>MATTVQLSDQSLRQLETLAIHTAHLIQPHGLVVVLQEPDLTISQISANCTGILGRSPEDLLGRTLGEVFDSFQIDPIQSRLTAGQISSLNPSKLWARVMGDDFVIFDGVFHRNSDGLLVCELEPAYTSDNLPFLGFYHMARAALNRLRQQANLRDFYDVIVEEVRRMTGFDRVMLHRFDENNHGDVIAEDKRDDMEPYLGLHYPESDIPQPARRLFIHNPIRVIPDVYGVAVPLTPAVNPSTNRAVDLTESILRSAYHCHLTYLKNMGVGASLTISLIKDGHLWGLIACHHQTPKVIPFELRKACEFFGRVVFSNISAQEDTETFDYRVQLAEHEAVLLDKMTTAADFVEGLTNHPDRLLGLTGSQGAAICFGEKLILVGETPDEKAVQYLLQWLENREVQDVFFTSSLSQIYPDAVNFKSVASGLLAIPIARHNFLLWFRPEVLQTVNWGGDPNHAYEATQEDGKIELHPRQSFDLWKEIVRLQSLPWQSVEIQSALALKKAIVNLILRQAEEHHHHHH[4x]

Phytochromes are red-light-sensitive biliprotein photoreceptors that control a variety of physiological processes in plants, fungi, and bacteria. In prototypical phytochromes, photoexcitation of the dark-adapted Pr parent state leads to chromophore isomerization at the methine bridge between rings C and D, followed by thermal relaxations and conformational changes in the protein, eventually generating the light-activated Pfr state. The underlying structural changes include movement of numerous side chains and sheet-to-helix restructuring of a tongue-like hairpin extension of the PHY-domain. Remarkably, the single substitution of conserved Tyr176 by His in cyanobacterial phytochrome Cph1 increases the fluorescence quantum yield from 2.4 to 14.5%.

In this work, we have addressed both issues on the basis of the crystal structure of the Y176H variant of the Cph1 photosensory module as Pr. Protomer A was modeled contiguously, whereas residues 453–465 (chain B), 73–80 (chain C), and 452–465 (chain D) could not be modeled due to sparse electron densities, probably reflecting local disorder. Thus, the overall PCB geometry was modeled as ZZZssa following the NMR and RR spectroscopic data as discussed in the following sections. Whereas the interactions of conserved Arg222 and Arg254 with the B-ring propionate are similar to those of the WT Pr (A-conformation), a drastic change is observed at the Tyr → His mutated 176 site and its neighbor Tyr203, corresponding to the Pfr-characteristic B-conformation. Even though the resolution of 3.7 Å is modest, refinement with the Pr-like A-conformation in this region resulted in substantial difference signals. The B-conformation involves concerted changes at Asp185, Leu201, His202, and finally, a “tryptophan swap”,2 where the space occupied by Trp450 in WT Pr is replaced by Trp478 and Phe475 in Y176H. Pfr-like structural features of Y176H also include the interaction between conserved Asp207 of the PASDIP motif and Ser474 of the PRxSF motif. By contrast, WT Pr showed widespread resonance splitting. These results suggest that the overall rigidity of the Pr chromophore in the binding pocket is greatly enhanced by the Y176H mutation. Thus, Y176H represents a mixture of a Pr-like chromophore configuration with a Pfr-like protein structure.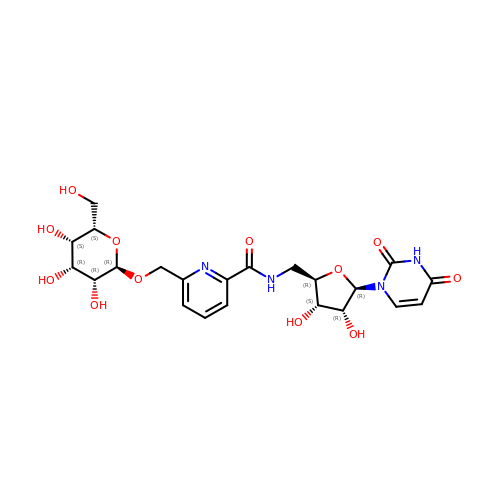6-(1-beta-D-Glucopyranosyloxymethyl)-N-(5'-deoxyluridine-5'-yl)picolinamide | C22 H28 N4 O12 | KPOTWZYLDCHCIG-MJELCBSSSA-N>MSAPYTLPELPYDYSALEPWISGEIMELHHDKHHAAYVKGANDALEQLAEAREKGDLSKVNLLQKNLAFNLAGHVNHTVFWPNLSPDGGDKPEGELGAAIDDAFGSFDAFRAHFSAAATGIQGSGWAILAWDILGQRLIIEQLYDHQGNLAAGSYPLLMLDMWEHAFYLQYKNVKADYVKAFWNVVNWADVAKRFEDARKVALG[2x]

Superoxide dismutases (SODs) are enzymes that catalyze the dismutation of the superoxide radical anion into O2 and H2O2 in a two-step reaction. They are ubiquitous to all forms of life and four different types of metal centers are detected, dividing this class of enzymes into Cu-/Zn-, Ni-, Mn-, and Fe-SODs. In this study, a superoxide dismutase from the thermophilic bacteria Thermobifida fusca (TfSOD) was cloned and expressed before the recombinant enzyme was characterized. The Mn- and Fe-SODs are structurally similar, normally appearing as 45 kDa homodimers where each monomer has an α-helical N-terminal domain and a C-terminal domain comprised of a three-stranded β-sheet surrounded by α-helices.

The crystal structure was solved by molecular replacement using the previously published crystal structure of Fe-PfSOD as a starting model. The structure was determined to 1.25 Å and refined to a Rwork of 11.5% (Rfree = 14.1%). The structure has a dimer in the asymmetric unit, and the biological tetramer is generated through the crystal symmetry. The metal center in both Fe- and Mn-SOD is bound by equivalent residues, being two histidines and one aspartate as equatorial ligands, a third histidine axially coordinated, and, most probably, a hydroxide as a fifth ligand completing a trigonal bipyramidal coordination polyhedron. This TfSOD structure was refined with an iron bound to His29, His77, Asp161 and H165 and two solvent molecules (W1, W2). Herein W1 has higher b-factor compared to the other ligands and Fe ion, thus W1 is less accurately defined. Even if the TfSOD is resolved to high resolution at 1.25 Å it is not possible to assign one of the solvent ligands (W1, W2) as hydroxide ion from the observed electron density, still, it is an option a hydroxide ion is present as reported for other SODs. In high resolution TfSOD crystal structure to 1.25 Å, the iron has octahedral coordinated, and the quaternary structure is tetrameric. To confirm the suggested Fe cofactor, EPR spectroscopy was conducted, giving a spectrum that was comparable to the EPR spectra of Fe-SODs from Desulfovibrio gigas, Themosynechocccus elongatus, Escherichia coli, and Methanobacterium thermoautotrophicum among other. The EPR envelope display g values of 4.90, 4.23 and 3.60 that are characteristic for a high spin ferric iron in the enzyme active site.> XXXXXX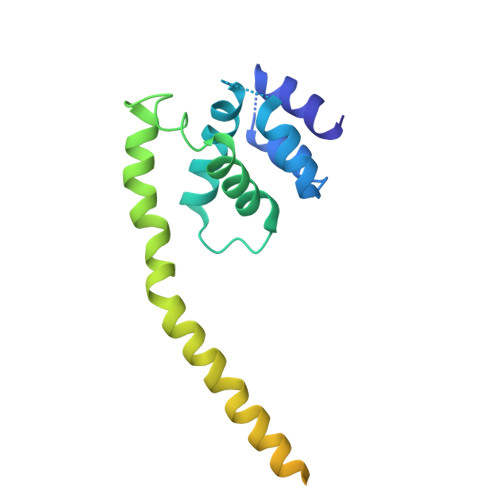XXXXXXXXXXXXXXXXXXXXXXXXXXXXXDHLSKIFLTISKSITQNPWNEENLLPLWLKWLLTLKSGELNSIKDKHTKKNCKHLKSALRSSEEILPVLLGIQGRLEMLRRQAKLREDLAQLSMQEGEDDEIEVIEHSNVISNPLQDQASPVEKLEPDSIVYANGESDEFVDASEYKD> GSTKERVERLCKSKELFEERLGLE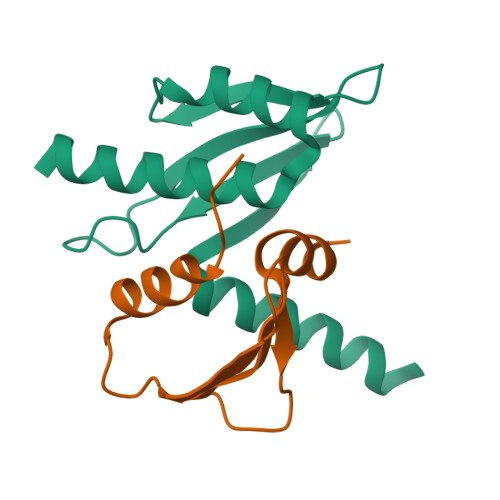IRRIHNEQLQFIFRHIDHKDPDKPYMFTLSINEQGDYEVTSCTPPLDCISEFQLKVRETNNFSAFIANIRKAFTALSFKQST;> GYEREDDGVPSAAYVTQLYYKISRIDWDYEVEPARIKGIHYGPDIAQPINMDSSHHSRCFISDYLWSLVPTAW2-amino-2-deoxy-6-O-phosphono-alpha-D-mannopyranose 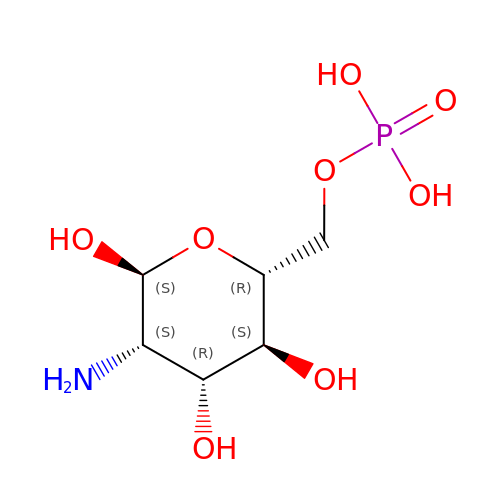| C6 H14 N O8 P | XHMJOUIAFHJHBW-RXRWUWDJSA-N> SPRA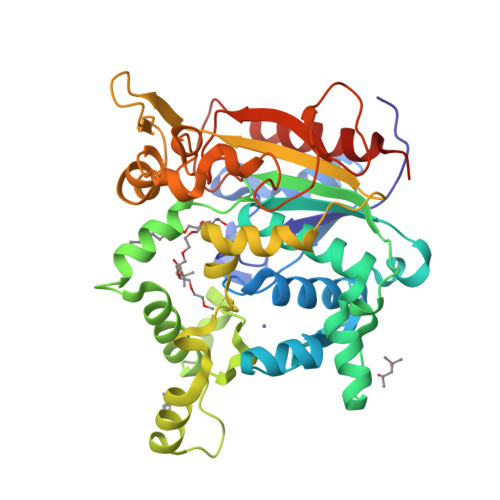NDAPIVLLHGFTGWGREEMLGFKYWGGVRGDIEQWLNDNGYRTYTLAVGPLSSNADRACEAYAQLVGGTVDYGAAHAAKHGHARFGRTYPGLLPELKRGGRVHIIAHSQGGQTARMLVSLLENGSQEEREYAKAHNVSLSPLFEGGHHFVLSVTTIATPHDGTTLVNMVDFTDRFFDLQKAVLKAAAVASNVPYTSQVYDFKLDQWGLRRQPGESFDHYFERLKRSPVWTSTDTARYDLSIPGAEKLNQWVQASPNTYYLSFSTERTHRGALTGNYYPELGMNAFSAVVCAPFLGSYRNEALGIDDRWLENDGIVNTVSMNGPKRGSSDRIVPYDGTLKKGVWNDMGTYNVDHLEVIGVDPNPSFDIRAFYLRLAEQLASLRP>[4x]SEKSAADQIVDRGMRPKLSGNTTRHNGAPVPSENISATAGPQGPNVLNDIHLIEKLAHFNRENVP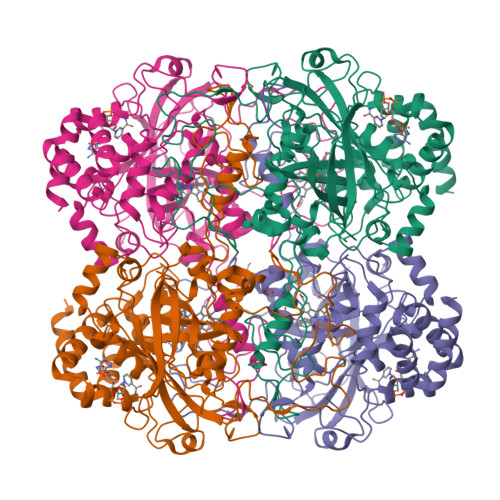ERIPHAKGHGAFGELHITEDVSEYTKADLFQPGKVTPLAVRFSTVAGEQGSPDTWRDVHGFALRFYTEEGNYDIVGNNTPTFFLRDGMKFPDFIHSQKRLNKNGLRDADMQWDFWTRAPESAHQVTYLMGDRGTPKTSRHQDGFGSHTFQWINAEGKPVWVKYHFKTRQGWDCFTDAEAAKVAGENADYQREDLYNAIENGDFPIWDVKVQIMPFEDAENYRWNPFDLTKTWSQKDYPLIPVGYFILNRNPRNFFAQIEQIALDPGNIVPGVGLSPDRMLQARIFAYADQQRYRIGANYRDLPVNRPINEVNTYSREGSMQYIFDAEGEPSYSPNRYDKGAGYLDNGTDSSSNHTSYGQADDIYVNPDPHGTDLVRAAYVKHQDDDDFIQPGILYREVLDEGEKERLADNISNAMQGISEATEPRVYDYWNNVDENLGARVKELYLQKKA> STDNAETGVIEAGNTDTDFSGELAAPGSNHTNVKFLFDRSRLLNVIKVLEKDAVFPRPFPTQEGAQQDDGYFCLLTPRPTVASRPATRFGLYANPSGSGVLANTSLDFNFYSLACFTYFRSDLEVTVVSLEPDLEFAVGWFPSGSEYQASSFVYDQLHVPFHFTGRTPRAFASKGGKVSFVLPWNSVSSVLPVRWGGASKLSSATRGLPAHADWGTIYAFVPRPNEKKSTAVKHVAVYIRYKNARAWCPSMLPFRSYKQKMLM;> GPIPTAPRENSLMFLSTLPDDTVPAYGNVRTPPVNYLPGEITDLLQLARIPTLMAFERVPE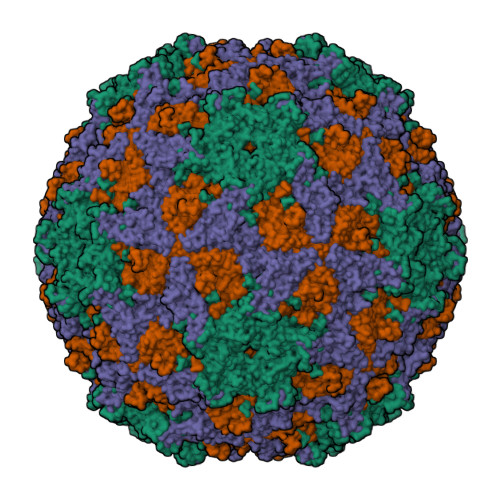PVPASDTYVPYVAVPTQFDDRPLISFPITLSDPVYQNTLVGAISSNFANYRGCIQITLTFCGPMMARGKFLLSYSPPNGTQPQTLSEAMQCTYSIWDIGLNSSWTFVVPYISPSDYRETRAITNSVYSADGWFSLHKLTKITLPPDCPQSPCILFFASAGEDYTLRLPVDCNPSYVFH;> DHNTEEMENSADRVTTQTAGNTAINTQSSLGVLCAYVEDPTKSDPPSSSTDQPTTTFTAIDRWYTGRLNSWTKAVKTFSFQAVPLPGAFLSRQGGLNGGAFTATLHRHFLMKCGWQVQVQCNLTQFHQGALLVAMVPETTLDVKPDGKAKSLQELNEEQWVEMSDDYRTGKNMPFQSLGTYYRPPNWTWGPNFINPYQVTVFPHQILNARTSTSVDVNVPYIGETPTQSSETQNSWTLLVMVLVPLDYKEGATTDPEITFSVRPTSPYFNGLRNRYTAGTDEEQ;> GNVQTTSKNDFDSRGNNGNMTFNYYANTYQNSVDFSTSSSASGAGPGNSRGGLAGLLTNFSGILNPLGYLK>MNNMNVIIADDHPIVLFGIRKSLEQIEWVNVVGEFEDSTALINNLPKLDAHVLITDLSMPGDKYGDGITLIKYIKRHFPSLSIIVLTMNNNPAILSAVLDLDIEGIVLKQGAPTDLPKALAALQKGKKFTPESVSRLLEKISAGGYGDKRLSPKESEVLRLFAEGFLVTEIAKKLNRSIKTISSQKKSAMMKLGVENDIAL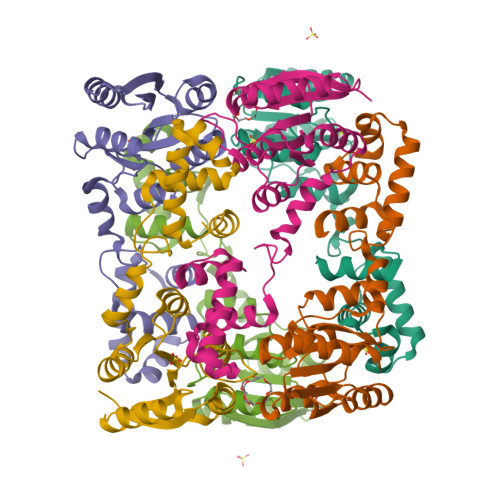LNYLSSVTLSPTDKE[6x]α-Methylacyl-CoA racemase in M. tuberculosis (MCR) has an essential role in fatty acid metabolism and cholesterol utilization, contributing to the bacterium’s survival and persistence. It catalyses the racemization of α-methyl-branched fatty acyl-CoAs, converting the (2S)-epimer to a near racemic mixture of the (2R)- and (2S)-epimers. The enzyme enables the conversion of α-methyl-branched fatty acids derived from cholesterol metabolism into forms that can be utilized by M. tuberculosis for growth and persistence within the host, a key component of M. tuberculosis pathogenesis. Within each active site, the large domain contributes the catalytic residues H126 (part of α-helix 3) and D156 (part of α-helix 5), while the small domain contributes a third catalytic residue, E241 (part of α-helix 9).

Crystals of the three MCR mutants H126A, D156A and E241A were obtained using identical conditions to those used with the wild-type enzyme and diffracted to 2.45, 1.64 and 1.85 Å resolutions, respectively. The overall structures for these single mutants were very similar to those of the wild-type structure, with small root-mean-squared deviation (RMSD) differences of 0.38, 0.37 and 0.38 Å for 693 Cα atoms of the H126A, D156A and E241A mutant structures being observed, respectively. The three mutants collectively had fewer hydrogen bond interactions; within the H126A, D156A and E241A mutants, 3, 5 and 5 interactions were observed, respectively. The active site of the E241A mutant stands out, as the relative positions of the active-site residues D156 and H126 are identical to the wild-type. These two active-site residues remain parallel to each other, and part of the PEG molecule is nestled in between them; consequently, most of the associated hydrogen bond interactions are retained. Within this mutant, the H126 residue is hydrogen-bonded to the peptide nitrogen atom of A241 through a water molecule, and due to this interaction, the movement of H126 gets restricted and it does not pivot away like E241 within the H126A mutant. This important structural water molecule within the E241A mutant active site resides where the functional group of the E241 side-chain was. However, the introduction of this structural water molecule does not replace all the hydrogen bonds lost in the active site. The rate-against-amount of enzyme plots show the expected enzyme-dependent increase in rate, while the specific activities calculated for wild-type, H126A, D156A and E241A were 46.4, 3.2, 18.5 and 12.2 µmol.min−1.mg−1. No significant change outside the enzymatic active site was observed in the three mutants, establishing that the diminution of catalytic activity is mainly attributable to disruption of the catalytic apparatus involving key hydrogen bonding and water-mediated interactions.

>[2x]MMAGPLSGLRVVELAGIGPGPHAAMILGDLGADVVRIDRPSSVDGISRDAMLRNRRIVTADLKSDQGLELALKLIAKADVLIEGYRPGVTERLGLGPEECAKVNDRLIYARMTGWGQTGPRSQQAGHDINYISLNGILHAIGRGDERPVPPLNLVGDFGGGSMFLLVGILAALWERQSSGKGQVVDAAMVDGSSVLIQMMWAMRATGMWTDTRGANMLDGGAPYYDTYECADGRYVAVGAIAPQFYAAMLAGLGLDAAELPPQNDRARWPELRALLTEAFASHDRDHWGAVFANSDACVTPVLAFGEVHNEPHIIERNTFYEANGGWQPMPAPRFSRTASSQPRPPAATIDIEAVLTDWDGGSGC>[5x]GMQMNN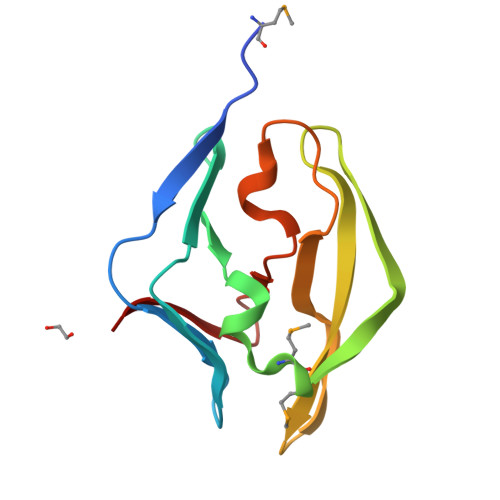HIRLRKAEGKWVIRTDSAVLGETLNAIELTEGSRDPVIYFPREDVAMVMFDKSEKVTACPLKGEASYYSIVGASGTLKDAAWSYESPKEGLEAIAGYLAFAPDCTKVGQY>MTELSPTALDPTELRSSLDKPFGTNRVIADDAMMADSITPAQYRYHHGSRVRPVNWNNIVDDKDLDVWNRLIANFWLPEKVPLSNDIPSWRSLTDLERKTTTRVFTGLTLLDTSQATIGELCQIEHARTEHEQAIYTNIAFMQSIHARSYSSIFSTLCSSEEIDEAYRWAVGNDVLQQRVTTVLCEYESEDPLKRKIAATMLSSLLLYAGFYLPLYFASRGKMMNTADMIRLILRDKAIHGYYSGYKFQRGLELRSENDKKNLEKFTMNLLDTLYDLEVEYSGQIYEGFDFHDDVFDFVRYNANKALM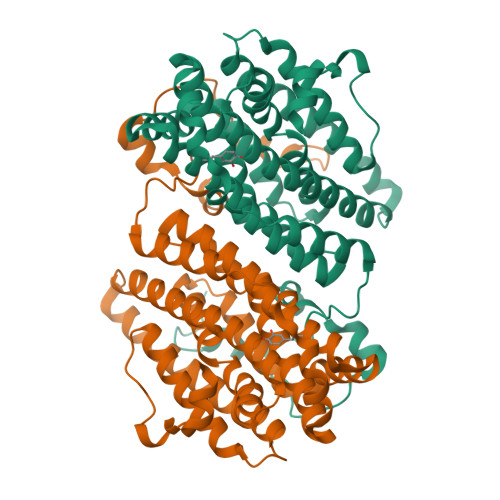NLGYPAKYSEEETHVSPEILAALSPAADENHDFFSGSGSSYIMGKSVETDDDDWDFLEHHHHHH[4x]> WMPINSIRVTVNGKRNDLLAQYYIPEDFLSTHAKCAPNTIPFETYVYGKYELEMKFVANGNKFQCGKVIISVKFDSYQADNINTGFQAALSRPHIMLDLSTNNEGVLKIPFRYHRAFVRNQTHKTATAGVRPG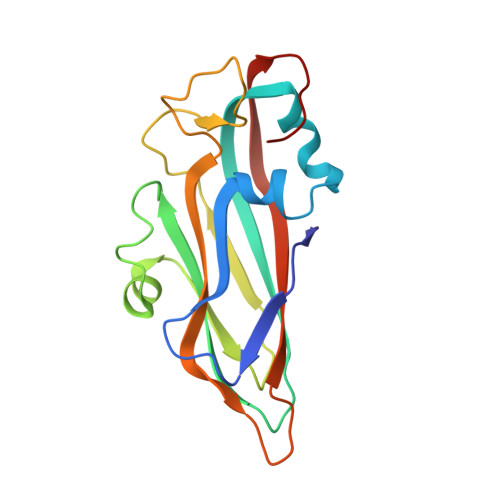KFASIYVQVLSPLQTGEGGANDMFIRPFYRYTRAEFAGMSYKVPLT In Kinetoplastids in general and Leishmania in particular, three PRTases are involved in the recycling of purine bases by the salvage pathway: hypoxanthine-guanine PRTase (HGPRT) (EC 2.4.2.8), adenine PRTase (APRT) (EC 2.4.2.7) and xanthine PRTase (XPRT) (EC 2.4.2.22). However, the Δhgprt/Δxprt double mutant L. donovani strain has less than 5% of the wild-type capacity to infect macrophages, establishing HGPRT and XPRT as essential for purine acquisition, parasite viability and infectivity in the mouse model. Leishmania HGPRT is an α/β protein with the known PRTase type I fold. It is composed of two domains: a core domain containing the PRPP binding site, and a hood domain that binds the purine base substrate.

The glycosomal HGPRT from Leishmania tarentolae in a catalytically active form purified and co-crystallized with a guanosine monophosphate (GMP) in the active site. The dimeric structure of HGPRT has been solved by molecular replacement and refined against data extending to 2.1 Å resolution. The N-terminal regions (residues 1–19), the active site flexible loops (residues 95–107 from chain A and 94–105 from chain B), and the C-terminal regions (residues 202–210) containing a glycosome target sequence, are absent from the model, since they could not be located by inspection of the experimental electron density maps. L. tarentolae HGPRT Loop III residues Asp129, Ser130, Ala131 and Thr133 interact with the GMP phosphate group. A flexible loop (loop II, residues 92–118), the function of which may be related to the formation of the transition state, comprises a region (residues 106–114) with good stereochemical and statistical values, which adopts different conformations in the two chains. In chain B, the polypeptide partially forms an α-helix (αL) similar to that in human HGPRT, while in chain A this helix is not observed and the polypeptide conformation resembles that found in T. cruzi HGPRT, Tritrichomonas foetus HGXPRT and E. coli HPRT. A loop (loop IV, residues 175–195) connects the β-strand β6 in the core domain to β8 in the hood-domain. This loop (IV) contains some of the residues that bind the base of GMP by hydrogen bonding with Val179 and Asp185 and by hydrophobic interaction with Phe178. An important contribution to the stabilization of GMP comes from Lys157 in strand β5, which makes two hydrogen bonds with the nitrogen base (atoms O6 and N7). Residues of the dimerization region are also involved in stabilizing the active site, particularly Arg191 (loop IV) and Lys66 (loop I), suggesting a structural explanation for the fact that Leishmania HGPRT has been found exclusively as a dimer in both the presence and the absence of GMP. Structural water molecules in each monomer (H2O1 and H2O18) stabilize the polar side chains of Thr37 and Tyr182 by hydrogen bonds that are found in a hydrophobic region formed by the Trp34, Val33, Phe71 and Phe78 side chains.

>MSNSVKSPSDHVGDVGRRNYPMSARTLVTQEQVWAATAKCAKKIAADYKDFHLTADNPLYLLCVLKGSFIFTADLARFLADEGVPVKVEFICASSYGSGVETSGQVRMLLDVRDSVENRHIMLVEDIVDSAITLQYLMRFMLAKKPASLKTVVLLDKPSGRKVDVLVDYPVITIPRAFVIGYGMDFAESYRELRDICVLKKEYYEKAESKL[2x]>[2x]SNAMMNQDI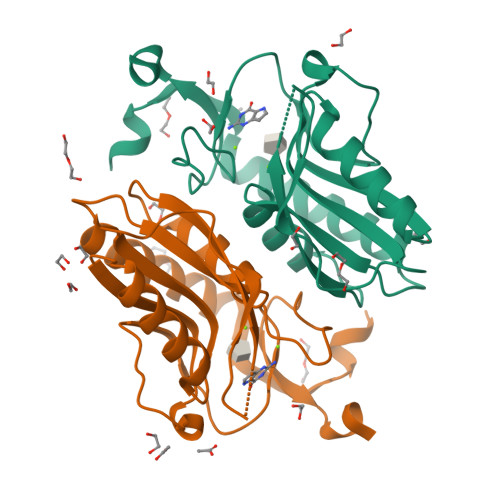EKVLISEEQIQEKVLELGAIIAEDYKNTVPLAIGVLKGAMPFMADLLKRTDTYLEMDFMAVSSYGHSTVSTGEVKILKDLDTSVEGRDILIVEDIIDSGLTLSYLVDLFKYRKAKSVKIVTLLDKPTGRKVDLKADYVGFTVPHEFVVGYGLDYKEQYRNLPYVGVLKPSVYSN> IVGGKVCPKGECPWQVLLLVNGAQLCGGTLINTIWVVSAAHCFDKIKNWRNLIAVLGEHDLSEHDGDEQSRRVAQVIIPSTYVPGTTNHDIALLRLHQPVVLTDHVVPLCLPERTFSERTLAFVRFSLVSGWGQLLDRGATALELMVLNVPRLMTQDCLQQSRKVGDSPNITEYMFCAGYSDGSKDSCKGDSGGPHATHYRGTWYLTGIVSWGQGCATVGHFGVYTRVSQYIEWLQKLMRSEPRPGVLLRAPFP;> ANAFLEELRPGSLERECKEEQCSFEEAREIFKDAERTKLFWISYSDGDQCASSPCQNGGSCKDQLQSYICFCLPAFEGRNCETHKDDQLICVNENGGCEQYCSDHTGTKRSCRCHEGYSLLADGVSCTPTVEYPCGKIPILEKRNASKPQGR;> GTTNTVAAYNLTWKSTNFKTILEWEPKPVNQVYTVQISTKSGDWKSKCFYTTDTECDLTDEIVKDVKQTYLARVFSYPAGNVESTGSAGEPLYENSPEFTPYLETNLGQPTIQSFEQVGTKVNVTVEDERTLVRRNNTFLSLRDVFGKDLIYTLYYWKSSSSGKKTAKTNTNEFLIDVDKGENYCFSVQAVIPSRTV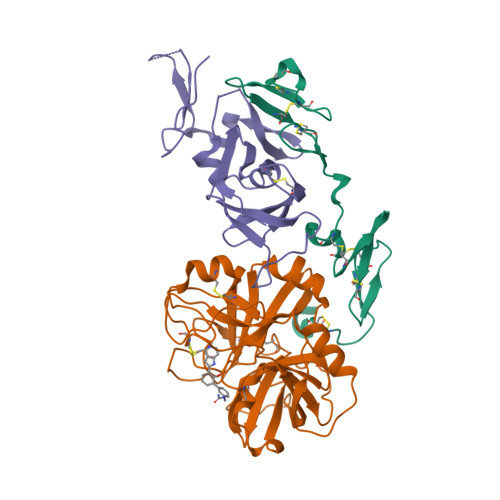NRKSTDSPVECMGQEKGEFRE>[4x]MAKDIGINSDPNSSSVDKLMKSSGVSNPTYTLVWKVWILAVTLYYAIRIPLTLVFPSLFSPLLPLDILASLALIADIPLDLAFESRRTSGRKPTLLAPSRLPDLLAALPLDLLVFALHLPSPLSLLSLVRLLKLISVQRSATRILSYRINPALLRLLSLVGFILLAAHGIACGWMSLQPPSENPAGTRYLSAFYWTITTLTTIGYGDITPSTPTQTVYTIVIELLGAAMYGLVIGNIASLVSKLDAAKLLHRERVERVTAFLSYKRISPELQRRIIEYFDYLWETRRGYEEREVLKELPHPLRLAVAMEIHGDVIEKVPLFKGAGEEFIRDIILHLEPVIYGPGEYIIRAGEMGSDVYFINRGSVEVLSADEKTRYAILSEGQFFGEMALILRAPRTATVRARAFCDLYRLDKETFDRILSRYPEIAAQIQELAVRRKELESSGLVPRGSVKHHHH

In order to address this void, we selected SthK, a prokaryotic cyclic nucleotide-modulated channel from Spirochaeta thermophila. We showed previously that SthK is activated by cyclic nucleotides and its activity is modulated by depolarizing voltages, making it more similar in this respect to CNG rather than HCN channels. Similar to the eukaryotic cyclic nucleotide-modulated ion channels whose structures were solved recently by cryo-EM (HCN1, TAX-4), the SthK channel is a functional tetramer and the structure can be divided in three layers as viewed from the membrane plane. SthK is a potassium selective channel, and displays a traditional potassium channel pore architecture where the selectivity filter, encoded by the TIGYGD signature sequence for potassium selection, is the same as that of KcsA and other potassium channels.

The apo structure adopts an architecture different from any of the existing CNG/HCN structures, which is expected, as it is the first apo, resting state structure of a member of the CNG channel family. We present here the high-resolution cryo-EM structures of SthK in the apo, cAMP-bound, and cGMP-bound states in lipid nanodiscs. This is, to our knowledge, the first apo, resting structure of a member of the CNG channel family. We will call this the ‘activated’ CNBD conformation. In all our full-length SthK structures, whether apo, or ligand-bound, the C-helix is swung away from the binding pocket (Figure 6D–E green), most similar to the only reported apo CNBD conformation of HCN2. We will call this the ‘resting’ CNBD conformation. Roughly half way down the membrane, in the middle of this cavity, the side chains of I215 pointing radially towards the pore axis, constrict the pore to a diameter of the size of a dehydrated potassium ion similar to what is seen in the HCN1 and LliK channels pore. Thus, it is possible that the gate in SthK is located at a previously unreported location, in the middle of the cavity, which is the second narrowest point in the permeation pathway, after the selectivity filter. Since the channel experiences a membrane potential of 0 mV on the EM grid, and the median value for voltage activation is about 85 mV, the voltage sensor is likely in the down, resting conformation in the SthK structure. Since these channels are in lipid nanodiscs, and we see these densities in each of the three structures at the same positions, we assigned them to lipid molecules binding specifically to SthK (POPG, since the nanodiscs were assembled with this lipid only). Conversely, the conformational change is less favored when less efficacious agonists are bound, so that most bound channels are closed. Our data shows identical, closed structures for the apo and inefficacious, partial agonist-bound SthK channels, which is consistent with the concerted gating model (the functional states - closed - that we solved with cryo-EM are indicated by dashed green circles in Figure 8E, top).The proteasome of the malaria parasite Plasmodium falciparum (Pf20S) is an advantageous drug target because its inhibition kills P. falciparum in multiple stages of its life cycle and synergizes with artemisinins. The 20S proteasome core particle is composed of two antechambers located between an α-ring and a β-ring and a catalytic chamber centrally located between two β-rings. Unfolded peptide substrates must pass through the antechamber before reaching the catalytic chamber for degradation. We recently developed a macrocyclic peptide, TDI-8304, that is highly selective for Pf20S over human proteasomes and is potent in vitro and in vivo against P. falciparum.

Using highly enriched Pf20S purified from Pf NF54 pellets, we determined the cryo-EM structure of the TDI-8304-bound complex at an average resolution of 2.18 Å. In the Pf20S–TDI-8304 structure, in addition to two anticipated TDI-8304 molecules in the two β5 subunits, there are four unexpected TDI-8304 molecules, two in the two β2 subunits, and two in the two antechambers near the β-annulus, in a pocket formed by subunits β3, β4, and α3. The EM densities of all six TDI-8304 molecules were well resolved for unambiguous atomic modeling. No TDI-8304 density was observed in any β1 catalytic pocket, even when the EM map was displayed at a low threshold. TDI-8304 binds to the β5 subunit with the P1 cyclopentyl group projecting into the S1 pocket and the P3 morpholino group inserting into the S3 pocket. The main chain of the cyclic peptide-like inhibitor binds to the substrate cleft in an antiparallel β-sheet mode, forming an extensive hydrogen bonding network with Ser21, Gly47, and Ala49 of β5 and the side chain of Asp153 of β6. The TDI-8304 pyrrolidinone forms two hydrogen bonds with the β6 Ser154 to further enhance the affinity. Importantly, TDI-8304 also makes extensive contact with several hydrophobic residues including Ala20, Met22, Met45, Gly48, and Ala49 of β5 and Phe135, Val155, and Cys159 of β6. The P5 pyrrolidinone has only a weak hydrogen bonding with β2 Glu22, as compared to the strong hydrophobic interactions with β5 Met22 and Phe135 and two hydrogen bonds with β6 Ser154 in the β5/β6 site. The macrocyclic ring of TDI-8304 fits snugly in an alcove formed by the α3, β3, and β4 subunits, with the P1 cyclopentyl and P3 morpholino groups partially exposed to the solvent in the antechamber.

>MVRPSQSMYDRHLTIFSPDGNLYQIEYAIKAVKNTNITSVGVKGENCAVIISQKKMATQYISQDKLLDYNNITNIYNITDEIGCSMVGMPGDCLSMVYKARSEASEFLYSNGYNVNAETLCRNICDKIQVYTQHAYMRLHACSGMIIGIDENNKPELFKFDPSGFCAGYRACVIGNKEQESISVLERLLEKRKKKIQQETIDEDIRNTTILAIEALQTILAFDLKASEIEVAIVSTKNRNFTQISEKEIDNYLTYIAERD[2x];>[2x]MADGEYSFSLTTFSPTGKLVQIEYALNRVSSSSPALGIRAKNGVIIATEKKSPNELIEENSIFKIQQISEHIGIVYAGMPGDFRVLLKRARKEAIRYSLQYGSEILVKELVKIIASIVQEFTQTGGVRPFGLSLLICGVDVYGYHLYQIDPSGCYFNWMATCVGKDYQNNMSFLEKRYNKDIEIEDAIHTAILTLKESYEGVLNEKNIEIGVAYDNKPFKILTQNEIKDYLIEIE;>[2x]MARRYDSRTTTFSPEGRLYQVEYALEAINNASITIGLITKDGVILGADKVFISKLIDKANNYEKIYKIDKHIFCGVAGLNADANILINQSRLYAQRYLYNYNEVQPVSQLVVQICDIKQSYTQYGGLRPYGVSFLIGGYDTKDGYQLYHTDPSGNYSGWFATAIGTNNLTASSVLKQEWKNDMTLEEGLLLALKTLAKSTDTEIPKSEKIELAYLTNKDGEVYQKYLTEKEIEELIKLYTQKYIKE;>[2x]MSYDRAITVFSPDGHLLQVEHALEAVKKGGCAVAIKSSNFAVLAVEKKNIPKLQNPKTTEKLIKLDEHNCLAFAGLNADARVLVNKTRLECQRYYLNMDEPAPVDYIAKYVAKVQQKFTHRGGVRPFGIATLIAGFKNNKEICIYQTEPSGIYAAWKAQAIGKNAKIVQEFLEKNYQENMEQKDCIFLALKAIFEVVELSSKNVEVALLTEKDLTFIEEQEINSMVELIDQERTKNNEQNE;>[2x]MFSTRSEYDRGVNTFSPEGRLFQVEYALGAIKLGSTAVGICVNDGVILASERRISSTLIEKDSVEKLLSIDDHIGCAMSGLMADARTLIDYARVECNHYKFIYNENINIKSCVELISELALDFSNLSDSKRKKIMSRPFGVALLIGGVDKNGPCLWYTEPSGTNTRFSAASIGSAQEGAELLLQENYKKDMTFEQAEILALTVLRQVMEDKLSTSNVEICAIKKSDQTFYKYNTDDISRIIDVLPSPVYPTIDMTA;>MYRNLYDTDNIIYSPEGRLYQVEYASEAIKQGTCAVAIKSKDYVVVSGLKKCISKLSFPQEKIFKIDDYIGISMSGITSDAKVLTKFMQNECLSHKFLYNENINIESLVRSVADKYQKNTQKSSKRAFGVGLMIAAYHNEPCIFETRPNGSYFEYDALSFGARSHASKTYLEKNLHLFEECSLEELILHCLKALKCSLSSESELTISNTALAVVGKNHPWQEISSLQLEEYLSKVKMDAEQEQVEENVQNEAN[2x];>[2x]MAGLSAGYDLSVSTFSPDGRLYQVEYIYKSINNNNTALCLECKDGIICCCINSNMDKNKMIKKNSYNRIYHVNNNIIITYSGFDGDARNIIDRARSEANTYYYNFHTNIPLHILVNRISLYIHAYTLYWHMRPFAASIIISSFNEKDKGDIYCIEPNGACYKYSGIVIGKNKEMFKTEIEKKDYKDINVRDAIEDIYKFILTSDDHMNKNNLQNLVNFSWICKESSYEFQNIHEEILTPALNKAVEYIEKLN;>TTIIGIIYDNGVMLACDSRTSSGTFISNKCSRKINRINENLYVCRSGASAHSQKIIEIIKHYCVSMKNENRKKGRFHEGETIYDETTYDEEIDIDSINYLDYNNNNDNNLVTKNKYFYEDKFNDYNPLVENVAHITKKIIYTNNNFLSCALIFGGYDKIKKQQLYAVNLNGSIIEKHDFAVSGSGSIYIQSYLQDKYKKFMTKKECFNLILNCVKYAMHNDNSSGGLIRIVNITKSFVEEFTVVNTQMNFQY[2x];>TTICGLVCQNAVILGADTRATEGPIVADKNCSKLHYISKNIWCAGAGVAGDLEHTTLWLQHNVELHRLNTNTQPRVSMCVSRLTQELFKYQGYKVCAIVLGGVDVNGPQLYGIHPHGSSCLLPFTALGSGSLNAMAVLEAKYRDNMTIEEGKNLVCEAICAGIFNDLGSGGNVDICVITKDSYQHIRPYKEPNMRLYHLPHPTIYPKGTTPILSEKIEYIKKFISVEDA[2x];>MGSIYNYNGGCVLGMSGSNCVAIACDLRLGANTFTTVSTKFSKIFKMNNNVYVGLSGLATDIQTLYEILRYRVNLYEVRQDAEMDVECFANMLSSILYSNRFSPYFVNPIVVGFKLKHYVDEEGEKKVNYEPYLTAYDLIGAKCETRDFVVNGVTSEQLFGMCESLYVKDQDENGLFETISQCLLSALDRDCISGWGAEVLVLTPEKIIKKKLKARMD[2x];>MDTLIGLRGNNFVVLAADTYSINSIIKLKNDDNTKFYDIHGNKCLLLGGSIGDRLQFGEFIRKNVHLYQYQNNTDMFVKSFAFFTRKNLAYYLRRNPFEVNCLIAGYDKKDGYQLYWCDYLSNMDSVNKGAHGYGAYLVSAILDKYYHENLTVDEALDIFKLCFEELKKRFLLTQINYELRIMYDNKVETQYVTV[2x];>[2x]TTTLAFKFKDGIIVAVDSRASMGSFISSQNVEKIIEINKNILGTMAGGAADCLYWEKYLGKIIKIYELRNNEKISVRAASTILSNILYQYKGYGLCCGIILSGYDHTGFNMFYVDDSGKKVEGNLFSCGSGSTYAYSILDSAYDYNLNLDQAVELARNAIYHATFRDGGSGGKVRVFHIHKNGYDKIIEGEDVFDLHYHYTNPEQKDQYVM;>MDLILYNDNLTEKKTEKENVIEHGRGFKRWYPYIDNGGTVIGLTGKDYVILAADTRLSLSYSIYTRFCPKISKLTDKCIIGSSGMQSDIKTLHSLLQKKIQLFVLEHSHYPDIHVIARLLCVILYSRRFFPYYAFNILAGVDENNKGVLYNYDSVGSYCEATHSCVGSGSQLILPILDNRVEQKNQLIKNTNFNLGDDINFVKDAITSATERDIYTGDKTLIYVIDKMGINVNTLDLKQD[2x];>MTLGPVVTGTSVIAIKYKHGIMIAADRKASYGSYAKFQNVERIFKINNKTVMGFSGELADAQYLHELLTRKNINNLSEKKRKEDMYTPQHYHSYVSRVFYVRKNRIDPLFNNIIIAGINSQKYDNNDDNVLLYTNKNNDDEQNEYKNNEEYKEIHKDDLYIGFVDMHGTNFCDDYITTGYARYFALTLLRDHYKDNMTEEEARILINECLRILYFRDATSSNFIQIVKVTSKGVEYEEPYILPCVLNSADYVYPSTLLPPAGCMW[2x]> YPFVE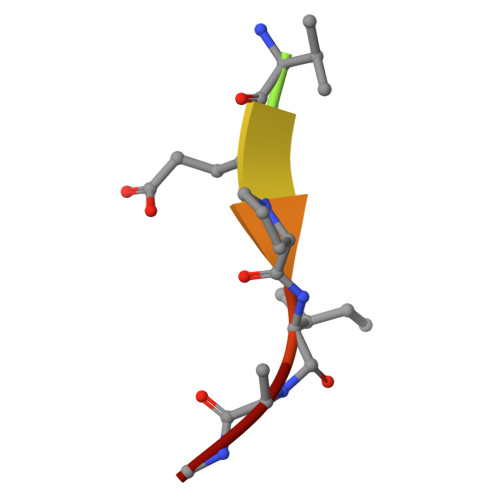PIKA> MKTINSVDTKEFLNHQVANLNVFTVKIHQIHWYMRGHNFFTLHEKHDDLYSEFGEQMDEVAER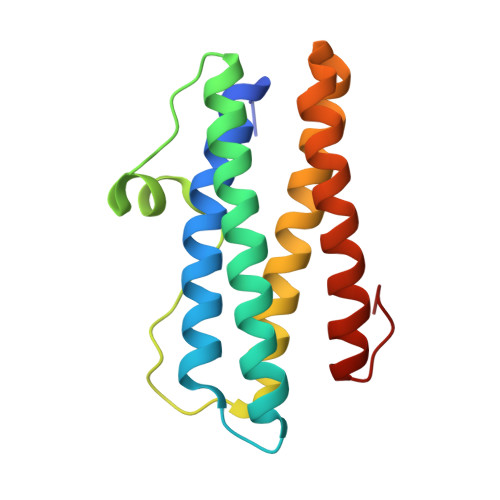LLAIGGSPFSTLKEFLENASVEEAPYTKPKTMDQLMEDLVGTLELLRDEYKQGIELTDKEGDDVTNDMLIAFKASIDKHIWMFKAFLGKAPLE> GEFEKLEVLEEWQSHIEGWEGSNIT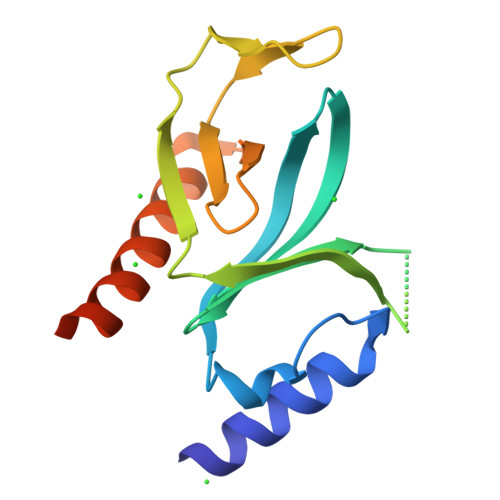DTCTEMLMCGVLLKISSGNIQERVFFLFDNLLVYCKRKHRRLKNSKASTDGHRYLFRGRINTEVMEVENVDDGTADFHSSGHIVVNGWKIHNTAKNKWFVCMAKTPEEKHEWFEAILKERERRKGLKLGMEQDTWVM> MSSLQSTRERVLGTPRRRYKV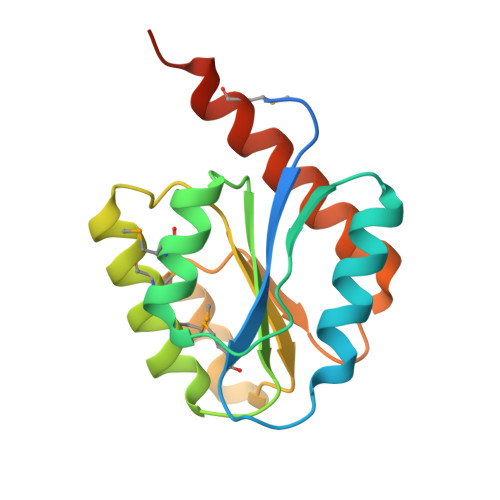LVAKMGLDGHDRGAKVVARALRDAGFEVVYTGLRQTPEQVAMAAVQEDVDVIGVSILNGAHLHLMKRLMAKLRELGADDIPVVLGGTIPIPDLEPLRSLGIREIFLPGTSLGEIIEKVRKLAEEKRMREEAEASEQVGQA> KKAVINGEQIRSISDLHQTLKKELALPEYYGENLDALWDALTGWVEYPLVLEWRQFEQ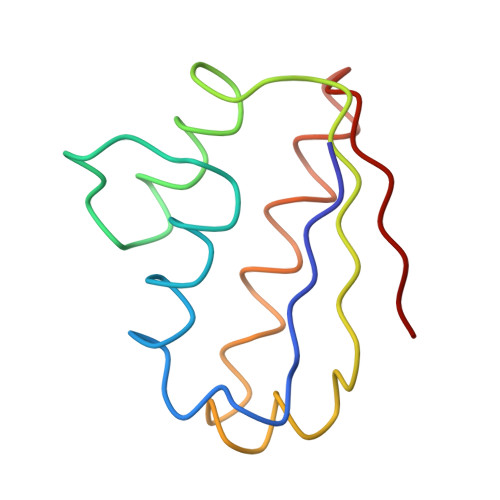SKQLTENGAESVLQVFREAKAEGADITIILS To make the 1D 1H-NMR method broadly applicable for the investigation of dynamic conformation change in both small proteins and large membrane protein complexes, we report the highly efficient and selective incorporation of TMSiPhe in proteins in Escherichia coli cells. The Key to the success of this method was the identification of a mutant Methanococcus jannaschii tyrosyl-tRNA synthetase (TyrRS) that exhibits high specificity toward 4-trimethylsilyl phenylalanine (TMSiPhe) in E. coli cells. The application of the genetic coding of TMSiPhe and its combination with the 1D 1H-NMR spectrometry for detection of conformational change in a biological system was named as DeSipher method, and is used for specific incorporation of Si into the desired protein. In particular, the low electronegativity of Si led to a uniquely low 1H chemical shift for CH3-Si (typically <0.55 ppm), which could be easily identified from the complicated 1H spectra of macro-biomolecules.

To investigate the molecular basis of the selective recognition of TMSiPhe by TMSiPheRS, we crystallized TMSiPheRS and analyzed the structures by X-ray crystallography. The crystal structures of TMSiPheRS alone and the complex of TMSiPheRS with TMSiPhe were determined at 1.8 Å and 2.1 Å, respectively. The 2Fo-Fc annealing omit map of the TMSiPheRS/TMSiPhe complex unambiguously assigned the electron density for TMSiPhe. Introduction of the TMS group significantly increased the volume of the amino-acid substrate by ~60%. To compensate for this substantial change in volume, three residues, namely, D158, I159, and V164, were replaced by the smallest amino-acid glycine, and Y32 and L65 were substituted by the relatively small residues H32 and V65, respectively. We then compared the crystal structure of the TMSiPheRS/TMSiPhe complex with that of apo TMSiPheRS. Compared with the structure of TMSiPheRS alone, we observed a dramatic 120-degree rotation of histidine 32 in response to TMSiPhe binding. Moreover, Leu162 rotated ~42 degrees to form hydrophobic interactions with the methyl groups of TMSiPhe. Altogether, G34, V65, Q70, F108, Q109, Y151, Q155, G158, G159, Q173, and H177 defined a hydrophobic pocket for the accommodation of and specific interactions with the phenyl ring and TMS group of TMSiPhe. These observations provided a structural basis for specific and efficient incorporation of TMSiPhe using evolved TMSiPheRS.

>[2x]MDEFEMIKRNTSEIISEEELREVLKKDEKSAHIGFEPSGKIHLGHYLQIKKMIDLQNAGFDIGIVLADLQAYLNQKGELDEIRKIGDYNKKVFEAMGLKAKYVYGSEFQLDKDYTLNVYRLALKTTLKRARRSMELIAREDENPKVAEVIYPIMQVNGGHYLGGDVAVGGMEQRKIHMLARELLPKKVVCIHNPVLTGLDGEGKMSSSKGNFIAVDDSPEEIRAKIKKAYCPAGVVEGNPIMEIAKYFLEYPLTIKRPEKFGGDLTVNSYEELESLFKNKELHPMDLKNAVAEELIKILEPIRKRLLEHHHHHH(2R)-2-AMINO-3,3,3-TRIFLUORO-N-HYDROXY-2-{[(4-PHENOXYPHENYL)SULFONYL]METHYL}PROPANAMIDE | C16 H15 F3 N2 O5 S | 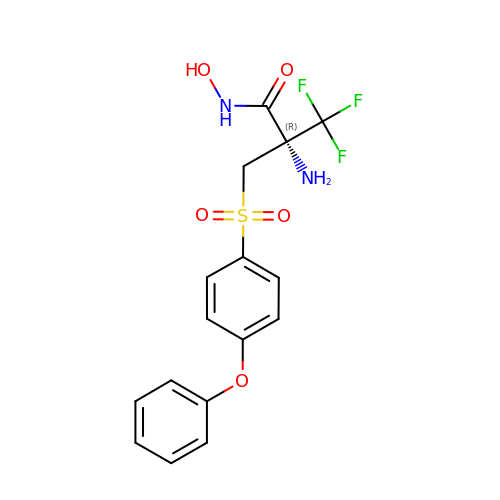MKRPIBSCGZAUCH-OAHLLOKOSA-N The A. baumannii outer-membrane transporter protein, BauA, that recognises this siderophore has itself been identified as a vaccine candidate. The siderophore is known to be bound from the medium by the integral outer-membrane BauA protein. BauA has the typical outer-membrane TonB-dependent transporter (TBDT) fold with a β-barrel formed by 22 antiparallel strands, several extracellular loops, and a plug domain folded inside of the barrel. Acinetobactin is synthesized as a precursor, preacinetobactin, which rearranges non-enzymatically and irreversibly at pH >7 to give acinetobactin.

Residues 33 to 703 of the protein are well defined in the electron density map, while the N-terminal region comprising the TonB box is missing, presumably because it is flexible. Compared to the other TBDTs, the extracellular loops of the β-barrel form a large open cavity bordered by mainly short and apolar amino acids giving large access to the loops NL1-NL3 of the plug domain. The asymmetric unit contains three monomers arranged around a threefold symmetry axis reminiscent of the porin arrangement and thus plausibly biologically meaningful. PISA, a computational assessment of oligomeric state in the crystal, suggests a trimer with a high degree of confidence. Biophysical methods (gel filtration and light scattering) do not support a trimeric assembly. Size Exclusion Chromatography coupled to Multi-Angle Light Scattering (SEC-MALS) analysis in C8E4 is consistent with monomer whilst native gel shows the protein runs more closely to a dimer; however, the detergent bound to the protein may increase the apparent weight suggesting a monomer in solution.

>GAMAVIDNSTKTLEQQTAQTNVAALPAITVKAEQDDTYAGGQVATSSNVGFLGSKKFLDTPFNTISYTDKYIEDKQAKDITEVIAATDPSIYTNGASGGWSENYYIRGYASSTNDMSMNGLFGITPFYRTSPEMFGRVEVLKGPSALLNGMPPAGSVGGTVNLVTKYAADEPFARLTTTYMSDAQFGGHVDVGRRFGENKEFGVRINGMYRDGDAAVNDQSKESRLFSLGLDWQGENARVFVDAYDALDHVDGVTRGVNVSTAVGIPKPPKADTLLSPDWGSVETKDKGAMIRGEYDFSDQLMAYAAYGQSTTEYKYNGASAGTITSSTGTLSSTLGQLAFDVDKKSADAGFKGKFETGSVKHQWVANATYYNHTQDDYSYRIIPGFSDPVITNIYDPNPNWGPKPEFTPPFLFHSTLSTSSFGLADTLSFAQDKVQLTLGLRHQTVKATSSVNTLPENAKSATTPGVALLIKATDKISVYANYIEGLTKGDQAPATASNPGEIFPPQKTKQQELGLKVDLGTFAHTLSAFEITKPSSYLDPSKLVNNLPTFVSDGEQRNRGIEWSFFGSPIEHVRLMGGFTYLDPELTKTKSGGNDGHTAVAVPKNQAKLGAEWDTQVAQGTLTLSGNINAVSKQYINAENTLSVPGRTLLDVGARYSTKVEDHPVTFRANIYNLTNKAYWAQPQLTNLALGAPRTYMLSVSYDF[3x]>MVFADSLFSDRFNRIDRLFSQLTGDTPVAATPAYDLQKRDANNYLLTVSVPGWKEEELEIETVGGNLNITGKHTEETVEDQTHWIYRGIRKADFQLSFSLPEHAKVNNAKLEQGLLLVEIYQEIPESEKPKKIAIES[6x]

Small Heat Shock Proteins (sHSPs) are ATP-independent chaperones which prevent irreversible protein aggregation by binding to misfolded substrate proteins. Most sHSPs exist as large oligomers which undergo drastic rearrangement or dissociation into dimers upon activation during stress, in order to execute their chaperone function. Aggregation Suppressing Protein A (AgsA), an sHSP from the pathogenic bacterium Salmonella enterica has been reported to form dynamic oligomers. In line with the current understanding of sHSP structure and function, our results show that in vivo, the wild type protein exists in an equilibrium between two oligomeric states: 18-mer and 24-mer.

Along with the wild type protein, we cloned different truncation constructs: AgsA:DelC lacking 9 residues at the C-terminus, double deletion AgsA:DD lacking 11 residues at the N-terminus and 9 residues at the C-terminus, and AgsA:His-DD, a hexa-histidine tagged double deletion construct. AgsA:DD formed symmetric 18-mers, an oligomeric assembly not reported previously. AgsA:DD crystallized in the R32 space group with 3 dimers in the asymmetric unit (ASU). The application of the crystallographic 3-fold axis yields a closed 18-mer, with a dimer lying along each side of a trigonal bipyramid. Thus, the 18-mer formed by nine dimers has a 32 symmetry. When this structure was used as a search model, an unambiguous MR solution of 3 dimers in the ASU was obtained, with clear and well-defined density for the β-sheets. The outer surface of the oligomer is charged, and its interior is hydrophobic. Long, continuous electron density is seen in the interior of the oligomer, which could account for the first 39 residues of the N-terminus. Though the IXI motifs in the C-termini of the 18-mer could not be defined for any monomer, the positioning of the monomers at inter-dimer interfaces indicates that the C-terminal regions are poised to form the hydrophobic interactions with the neighbouring β4–β8 clefts.>[4x]MARIRDVQGDITEFQGDAIVNAANNYLKLGAGVAGAILRKGGPSIQEECDRIGKIRVGEAAVTGAGNLPVRYVIHAAVLGDEPASLETV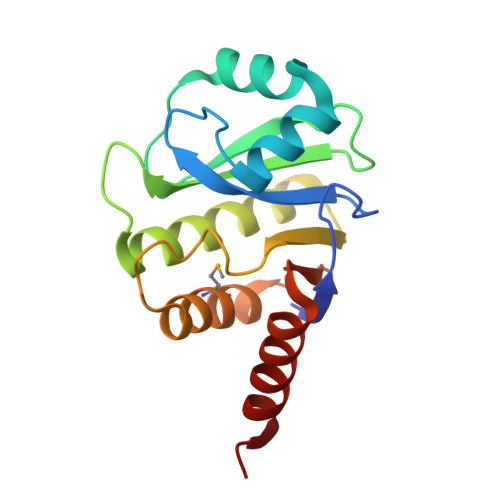RKATKSALEKAVELGLKTVAFTALGAWVGGLPAEAVFRVMFEEIKKAPDTLEVTGVHGTEKSAEAGRRATLEHHHHHH> MGSSKPLKGFVICCTSIDLKQRTEISTKATKLGAAYRSDFTKDVTHLIAGDFDTPKYKFAAKSRPDIKIMSSEWIPVLYESWVQGEDLDDGLLVDKHLLPTLFKCRVCLTNIGQPERSRIENYVLKHGGTFCPDLTRDVTHLIAGTSSGRKYEYAL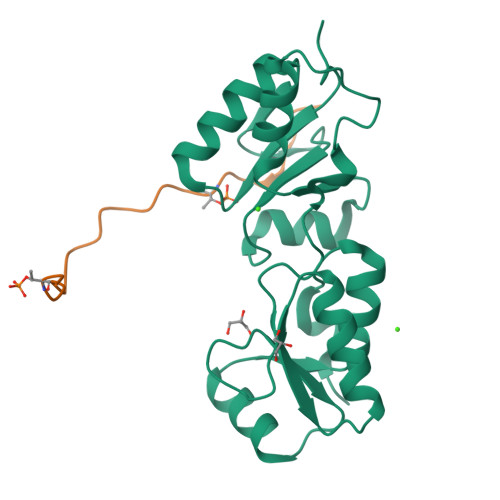KWKINVVCVEWLWQSIQRNAVLEPQYFQLD;> GYDSILVQATPRKSSSVITELPDTPIKMNS> QTVGVHSIVQQLHRNSIQFTDGYEVKEDIGVGSYS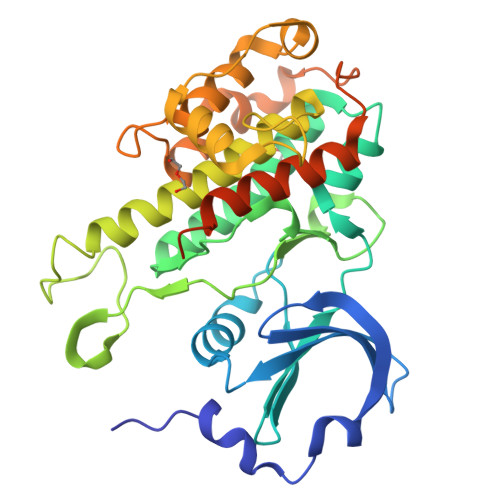VCKRCIHKATNMEFAVKIIDKSKRDPTEEIEILLRYGQHPNIITLKDVYDDGKYVYVVTELMKGGELLDKILRQKFFSEREASAVLFTITKTVEYLHAQGVVHRDLKPSNILYVDESGNPESIRICDFGFAKQLRAENGLLMTPCYTANFVAPEVLERQGYDAACDIWSLGVLLYTMLTGYTPFANGPDDTPEEILARIGSGKFSLSGGYWNSVSDTAKDLVSKMLHVDPHQRLTAALVLRHPWIVHWDQLPQYQLNRQDAPHLVKGAMAATYSALNRNQSPVLEPVGRSTLAQRRGIKKITSTAL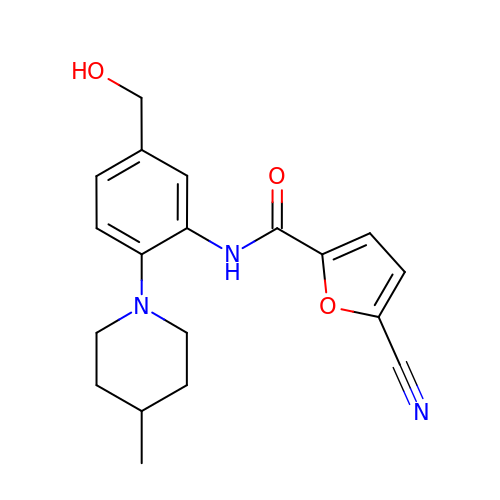5-CYANO-FURAN-2-CARBOXYLIC ACID [5-HYDROXYMETHYL-2-(4-METHYL-PIPERIDIN-1-YL)-PHENYL]-AMIDE | C19 H21 N3 O3 | NNPCFFIJVKYGHR-UHFFFAOYSA-N> MVKLDRYIGVTVFVAILAVLGVILGLALLFAFIDELNDISASYGIGDALRFIFLTAPRRAYDMLPMAALIGCLVGLGTLASNSELTIMRAAGVSLSRIVWAVMKPMLVLMLAGILVGEYVAPWTENIAQSGRALAQGGGDSQSSKRGLWHRQGREYIHINAVQPNGVLYGVTRYRFDEQRGLESASFAKRARFETDHWQLEEVTTTLLHPREKRSEVVKLPTERWDAQLSPQLLNTVVMEPEALSISGLWQYIHYLADQGLNNNRYWLAFWTKVLQPLVTAALVLMAISFIFGPLRSVTLGQRIFTGVLVGFVFRIAQDLLGPSSLVFDFPPLLAVVIPA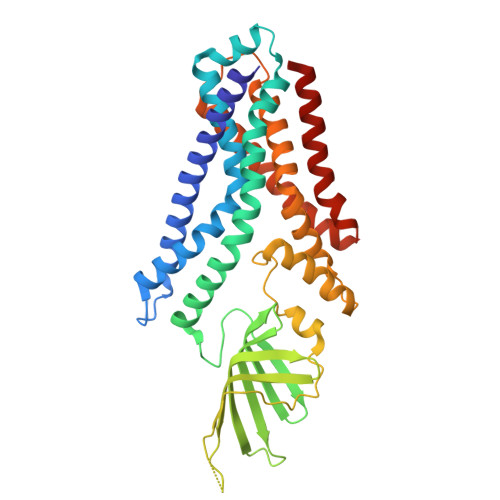SICALAGVWLLRRAG> MHHHHHHHDGTENPIHDRTSDYHKYLKVKQGDSDLFKLTVSDKRYIWYNPDPKERDSYECGEIVSETSDSFTFKTVDGQDRQVKKDDANQRNPIKFDGVEDMSELSYLNEPAVFHNLRVRYNQDLIYTYSGLFLVAVNPFKRIPIYTQEMVDIFKGRRRNEVAPHIFAISDVAYRSMLDDRQNQSLLITGESGAGKTENTKKVIQYLASVAGRNQANGSGVLEQQILQANPILEAFGNAKTTRNNNSSRFGKFIEIQFNSAGFISGASIQSYLLEKSRVVFQSETERNYHIFYQLLAGATAEEKK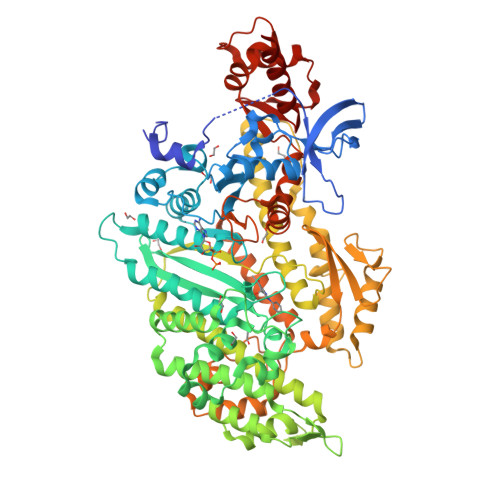ALHLAGPESFNYLNQSGCVDIKGVSDSEEFKITRQAMDIVGFSQEEQMSIFKIIAGILHLGNIKFEKGAGEGAVLKDKTALNAASTVFGVNPSVLEKALMEPRILAGRDLVAQHLNVEKSSSSRDALVKALYGRLFLWLVKKINNVLCQERKAYFIGVLDISGFEIFKVNSFEQLCINYTNEKLQQFFNHHMFKLEQEEYLKEKINWTFIDFGLDSQATIDLIDGRQPPGILALLDEQSVFPNATDNTLITKLHSHFSKKNAKYEEPRFSKTEFGVTHYAGQVMYEIQDWLEKNKDPLQQDLELCFKDSSDNVVTKLFNDPNIASRAKKGANFITVAAQYKEQLASLMATLETTNPHFVRCIIPNNKQLPAKLEDKVVLDQLRCNGVLEGIRITRKGFPNRIIYADFVKRYYLLAPNVPRDAEDSQKATDAVLKHLNIDPEQYRFGITKIFFRAGQLARIEEAREQRLESNE>AMALEQALQAARRGDLDVLRSLHAAGLLGPSLRDSLDALPVHHAARSGKLHCLRYLVEEVALPAVSRARNGATPAHDAAATGYLSCLQWLLTQGGCRVQEKDNSGATVLHLAARFGHPDVVKWLLYQGGANSAITTDTGALPIHYAAAKGDLPSLKLLVGHYPEGVNAQTNNGATPLYLACQEGHLEVTKYLVQECSADPHLRAQDGMTPLHAAAQMGHNPVLVWLVSFADVSFSEQDHDGATAMHFAASRGHTKVLSWLLLHGAEISQDLWGGTPLHDAAENGELECCQILAVNGAGLDVRDH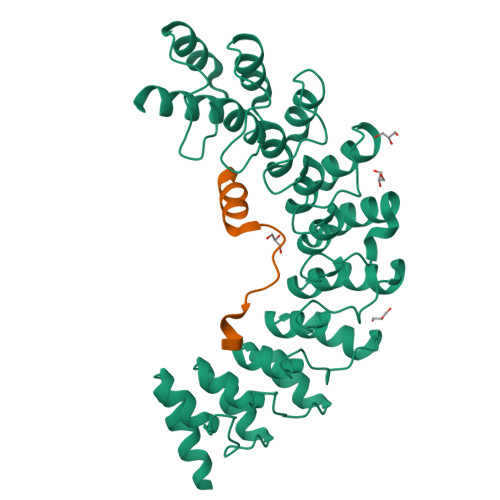DGYTAADLAEFNGHTHCSRYLRTVQTLSLEHRVLSRDQSMDLEAKQLDS[2x];>QKQRAPRRRCQQPKMLSSPEDTMYYNQLNGTLEYQG[2x]> SSGLPNTKRRIRDPFWRRSGWWRWRQQEVKAMNRSRAFRRHLFPRFTTETVSFVDAAEAEAKRFKEIVAETGRYPGQTVNFFVPKVEGAKLDPFAALPSRQKRLKLRRKAVREAEEAEKAREDADFVWRGKGGGRVWEERKANIPLGKKKLLLYCTIIKGLQITDAIDWLSSLCLHRVN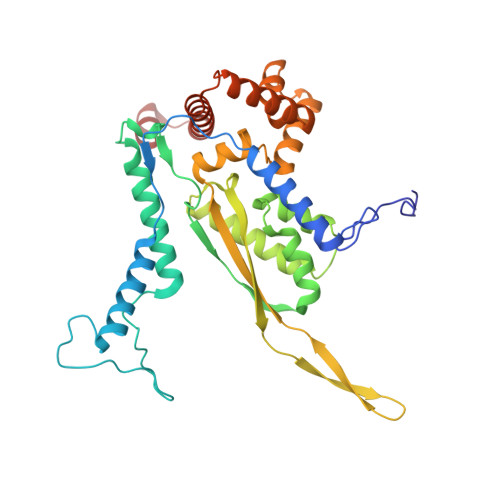YLLNLLNASRKKIHEQGGDISRVYVESYMLNIQGQIKRPQFRLRMVNLIKTWKFAVVLRFREYPMDEYFHKLFILKHVPRSLTTDMRLALAGQRVGLHAVRDWYPFLDSKTRFFHRKRLKWLDRTRQFDYCLARRVFKSKYEENCRRRKIQVLQARGASDAVIEEAN> MGSDKIHHHHHHVEKNLLRSALKIFEKKDLSLLAYSGRSIFESKDSGLKPVVELFKRFDNLEGSLVIDKMVGKAAASFLLK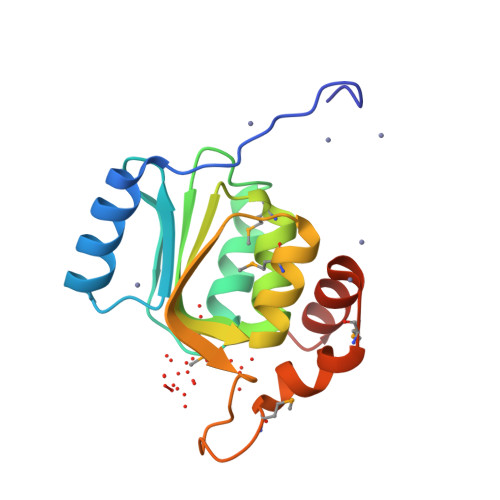MKPDHIHAKVISKPALKLMNEYGQSFSYDEKIPFVLGKDGKSMCPFEKLVLEMDDPEEIIRIVLSKFTSL> AMPLDAGGQNSTQMVLAPGASIFRCRQCGQTISRRDWLLPMGGDHEHVVFNPAGMIFRVWCFSLAQGLRLIGAPSGEFSWFKGYDWTIALCGQCGSHLGWHYEGGSQPQTFFGLIKDRLAEGPAD

Ito et al. showed that cereblon associates with damaged DNA binding protein 1 (DDB1) to act as a substrate receptor for the DDB1/cullin4 E3 ubiquitin ligase complex. In mammals, cereblon has a LON domain and a C-terminal thalidomide binding domain. However, homologs of the latter, also termed the CULT domain, are further found in animals and bacteria as single-domain proteins, that have all essential residues of the thalidomide binding site conserved. Architecturally, the thalidomide binding domain is a member of the β-tent fold, which consists of two antiparallel beta sheets that are oriented at an approximately right angle and pinned together at the top via a structural zinc ion.

We now obtained a new, trigonal crystal form of MsCI4•thalidomide that yielded a dataset with a resolution of 1.2 Å. The crystals contain one monomer in the asymmetric unit (ASU) in space group P3221, which has the same conformation as in all other known co-crystal structures of MsCI4. This structure superimposes closely with the 3 other monomers of MsCI4•thalidomide from the orthorhombic crystal form and the 2 further new MsCI4•thalidomide monomers described below. However, between all structures, there is a significant difference in the conformation of the thalidomide molecule: while the glutarimide moieties superimpose tightly, the phthaloyl moieties protruding from the binding pocket differ in their orientation by up to 13°. This angular freedom is especially apparent in the atomic resolution electron density. An obvious rationale for this conformational freedom lies in the lack of specific interactions of the phthaloyl moiety with the protein.>[4x]MKFSNITIKNFRNFEKVNINLDNKNVIFGMNDIGKTNFLYALRFLLDKEIRKFGFNKSDYHKHDTSKKIEIILTLDLSNYEKDEDTKKLISVVKGARTSANADVFYIALESKYDDKELYGNIILKWGSELDNLIDIPGRGNINALDNVFKVIYINPLVDLDKLFAQNKKYIFEESQGNESDEGILNNIKSLTDQVNQQIGEMTIIKGFQQEITSEYRSLKKEEVSIELKSEMAIKGFFSDIIPYIKKDGDSNYYPTSGDGRRKMLSYSIYNYLAKKKYEDKIVIYLIEEPEISLHRSMQIALSKQLFEQSTYKYFFLSTHSPELLYEMDNTRLIRVHSTEKVVCSSHMYNVEEAYGSVKKKLNKALSSALFAERVLLIEGPSEKILFEKVLDEVEPEYELNGGFLLEVGGTYFNHYVCTLNDLGITHIIKTDNDLKSKKGKKGVYELLGLNRCLNLLGRENLDEITIDIPEDIKGKKKKERLNERKKEIFKQYKNEVGEFLGERIYLSEIDLENDLYSAIGESMKRIFENEDPVHYLQKSKLFNMVELVNNLSTKDCFDVFEHEKFACLKELVGSDR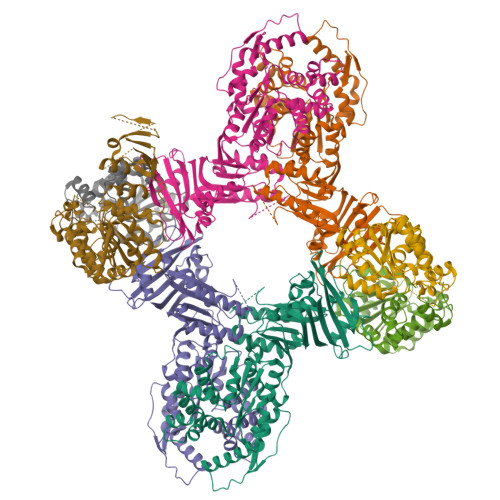G;>[4x]MSREQIIKDGGNILVTAGAGSGKTTILVSKIEADLKENKTHYSIAAVTFTNKAAKEIEGRLGYSSRGNFIGTNDGFVESEIIRPFIKDAFGNDYPDNFTAEYFDNQFASYDKGLQVLKYQNILGTYSNPKKNFKFQLALDILKKSLVARQYIFSKYFKIFIDEYQDSDKDMHNLFMYLKDQLKIKLFIVGDPKQSIYIWRGAEPENFNGLIENSTDFNKYHLTSNFRCCQDIQNYSNLFNEETRSLIKEKNEVQNVISIADDMPISDILLKLTEEKQVLNIEAELVILVRRRNQAIEIMKELNEEGFNFIFIPQTPLDRATPNATLLKEVIKYVKNDRYSIYDLAAEIVGNLSSREIKEIQKIINELLVPNINQVLINQVLINLFAKLEITLDTREITAFTEVMMTNEFDIAFDTNEYLHKIFTVHSAKGLEFNQVIITASDYNVHYNRDTNEHYVATTRAKDKLIVIMDNKKYSDYIETLMKELKIKNIIKSI> MTGSNSHITILTLNINGLNSAIKRHRLASWIKSQDPSVCCIQETHLTCRDTHRLKIKGWRKIYQANGKQKKAGVAILVSDKTDFKPTKIKRDKEGHYIMVKGSIQQEELTILNIYAPNTGAPRFIKQVLSDLQRDLDSHTLIMGAFNTPLSTLDRSTRQKVNKDTQELNSALHQADLIDIYRTLHPKSTEYTFFSAPHHTYSKIDHIVGSKALLSKC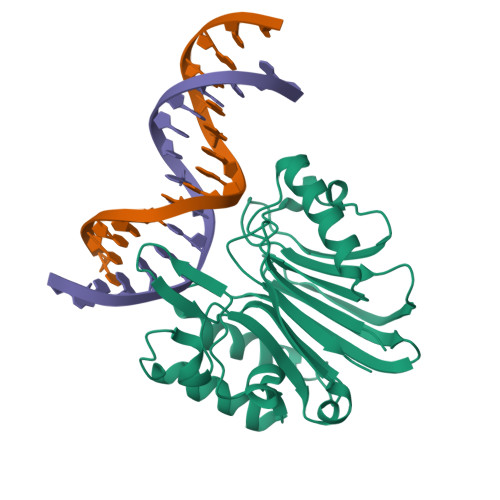KRTEIITNKLSDHSAIKLELR>GSHMNINKQSPIPIYYQIMEQLKTQIKNGELQPDMPLPSEREYAEQFGISRMTVRQALSNLVNEGLLYRLKGRGTFVSKPKMEQALQGLTSFTEDMKSRGMTPGSRLIDYQLIDSTEELAAILGCGHPSSIHKITRVRLANDIPMAIESSHIPFELAGELNESHFQSSIYDHIERYNSIPISRAKQELEPSAATTEEANILGIQKGAPVLLIKRTTYLQNGTAFEHAK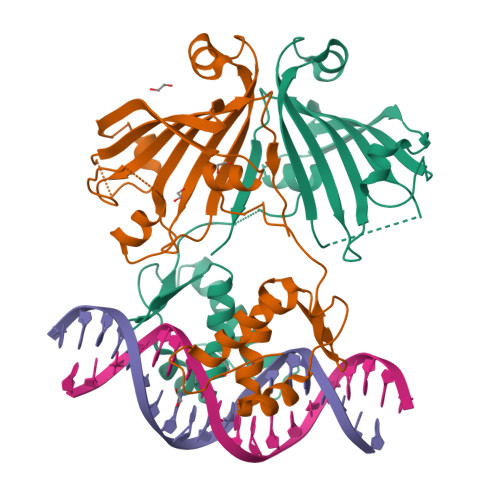SVYRGDRYTFVHYMDRLS[2x]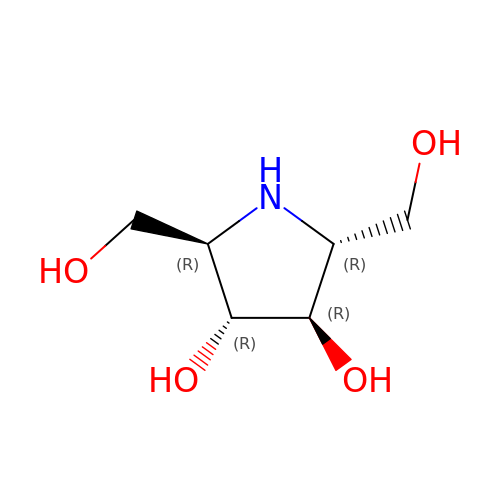2,5-DIDEOXY-2,5-IMINO-D-MANNITOL | C6 H13 N O4 | PFYHYHZGDNWFIF-KVTDHHQDSA-N Here, we focus on the ectoine hydroxylase, the enzyme that forms (4S,5S)-2-methyl-5-hydroxy-1,4,5,6-tetrahydropyrimidine-4-carboxylic acid from the precursor ectoine through a region-selective and stereospecific hydroxylation reaction. The EctD-mediated hydroxylation of (4S)-ectoine to (4S,5S)-5-hydroxyectoine requires O2 and 2-oxoglutarate as co-substrates, thereby forming CO2, succinate, and 5-hydroxyectoine. The catalytically critical iron is coordinated by the side chains of a conserved H×D/E…H motive, the so-called 2-His-1-carboxylate facial triad.

In addition, the crystal structure of the EctD protein from the salt tolerant moderate halophile V. salexigens in its iron-free form was solved, thereby allowing for the first time an assessment of the structural consequences of the binding of the active-site iron on the overall fold of the ectoine hydroxylase. However, after analyzing the iron content of this strongly overproduced EctD enzyme preparation, it became apparent that most of the isolated proteins did not contain an iron molecule; the iron content of the EctD protein solution dropped to 0.1–0.2 mole iron per 1 mol of EctD, rendering the enzyme largely inactive. Upon addition of Fe2+ ions prior to the enzyme activity measurements, we observed that the activity returned to levels observed before, indicating that the missing iron catalyst in the purified EctD protein can be restored after the protein has adopted its native cupin barrel fold. The cell constants and the space-group were identical to the structure of the iron-bound EctD, suggesting that the apo-EctD protein crystalized in a manner similar to that found in the iron bound form. After solving the new crystal structure of the EctD protein, it became apparent that the iron ligand was lacking, as evidenced by the missing pronounced electron density that is present in the iron-bound EctD crystal structure. Otherwise, the apo- and the iron-bound forms are almost identical, as indicated by the RMSD value of 0.34 Å over 280 Cα atoms. In the V. salexigens EctD protein, the iron ligand is bound via interaction with two histidine side-chains, His-146 and His-248, and the side-chain of Asp-148. Interestingly, in the apo-structure of EctD, two water molecules populate the iron-binding site formed by the 2-His-1-carboxylate facial triad. This keeps the side chains of the His-146, His-248 and Asp-148 in an orientation very similar to that observed in the iron-bound EctD crystal structure. Hence, the EctD apo-protein exists in a form that is pre-set to incorporate the iron catalyst.

> MEDLYPSRQNNQPKILKRKDPVIYTDRSKDNQAPITKEQLDSYEKNGFLQIKNFFSEDEVIDMQKAIFELQDSIKDVASDKVIREPESNDIRSIFHVHQDDNYFQDVANDKRILDIVRHLLGSDVYVHQSRINYKPGFKGKEFDWHSDFETWHVEDGMPRMRAISVSIALSDNYSFNGPLMLIPGSHNYFVSCVGETPDNNYKESLKKQKLGVPDEESLRELTRIGGGISVPTGKAGSVTLFESNTMHGSTSNITPYPRNNLFMVYNSVKNRLVEPFSGGEKRPEYIAVREKQPVYSAVNSAWSHPQFEK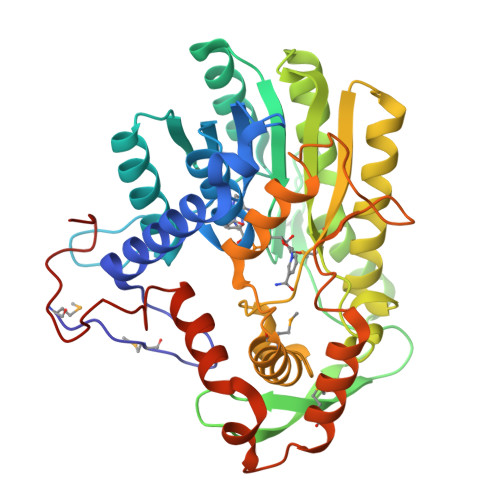>[16x]MIVKPMVRNNICLNAHPQGCKKGVEDQIEYTKKRITAEVKAGAKAPKNVLVLGCSNGYGLASRITAAFGYGAATIGVSFEKAGSETKYGTPGWYNNLAFDEAAKREGLYSVTIDGDAFSDEIKAQVIEEAKKKGIKFDLIVYSLASPVRTDPDTGIMHKSVLKPFGKTFTGKTVDPFTGELKEISAEPANDEEAAATVKVMGGEDWERWIKQLSKEGLLEEGCITLAYSYIGPEATQALYRKGTIGKAKEHLEATAHRLNKENPSIRAFVSVNKGLVTRASAVIPVIPLYLASLFKVMKEKGNHEGCIEQITRLYAERLYRKDGTIPVDEENRIRIDDWELEEDVQKAVSALMEKVTGENAESLTDLAGYRHDFLASNGFDVEGINYEAEVERFDRILEHHHHHH> MSLTINVGLLVDETGPTSDVGKGYSLGAELAFKYFNEKGIYTKDGVRVNINYIKRDYAYNPTTAEEYYREFRDRYGVIAIIGWGTADTEKLSDQVDTDKITYISASYSAKLLVKPFNFYPAPDYSTQACSGLAFLASE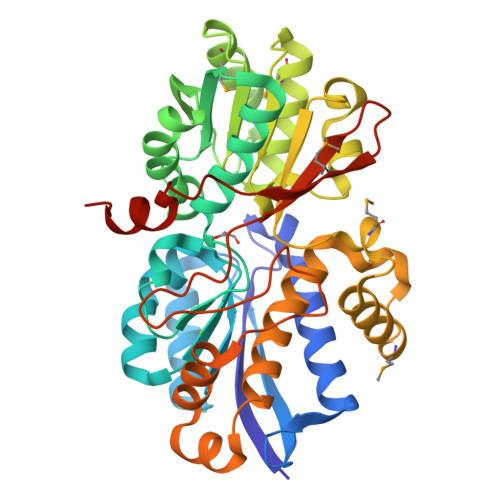FGQGKLALAYDSKVAYSRSPIGAIKKAAPSLGLQVVGDYDLPLRATEADAERIAREMLAADPDYVWCGNTISSCSLLGRAMAKVGLDAFLLTNVWGFDERSPQLIGEGGYGKVFGISPFIYPMFGQDVEGIQTIFEAARMNGVSEDQINLRVVQGFVNVWLLIKAIESVTSQDLQERGGEALKEALEANTFDLGGITADTIDYEPGFHLAYRKVFIIKLGENGELQLMGKFEAPSQVDCARYTIEEGHHHHHH> WKEIKFEFDTIDPADSFSGASPERKAAVALRSLFTFVAARVVLEQLQGPGGPETTYNQQAYLDLMDFLGTPMKGDGGDEWMAAVMRKNHALALRLMEVREAYLDEFEWGKTMEMASRETREA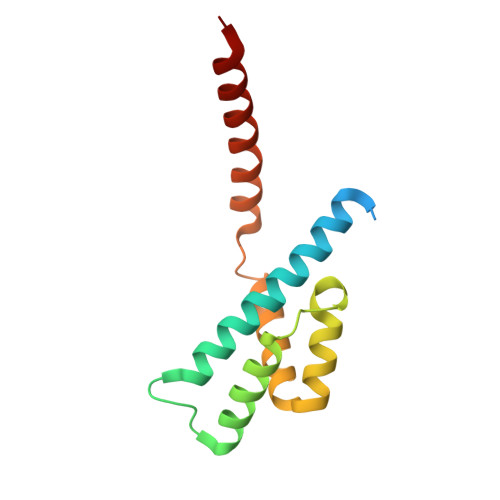NTRLMRAAAM>[2x]SNAMAVKDALRFPPTDVTPIFDLFRGNFATELLAASVAHLHVFDILNESPLSLDELQRRLVLSERATQVLVTGLCAMQLLTKRLAGEIDLTPLARNHLVTTSPFSVGGYIS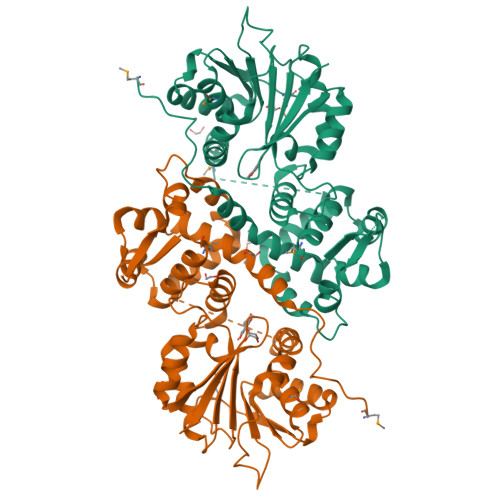LAAQSAGTLALVERLKSDRPEGAESEQGAAFIFREGSESAMDREDSARFLTLSLAGRAWNVAPRFADVLPAGQPGKILKDNSGSSGRVLLDVAGGSGIYTMAVLQKYPTWRGIIFDRPEVLKIAAELAEQTGVRDRLELHAGDMWVDPFPPADDILLSNVLHDWDRPQCARLVAKATSGLPEGGRLLIHDVLLNSDLTGPLEIALYSLALFSLTEGRAYSLEEYRGWIAGADLKYVDCIPTSAHGHLILSEKV3,3'-(2,4-diaminopteridine-6,7-diyl)diphenol | C18 H14 N6 O2 | 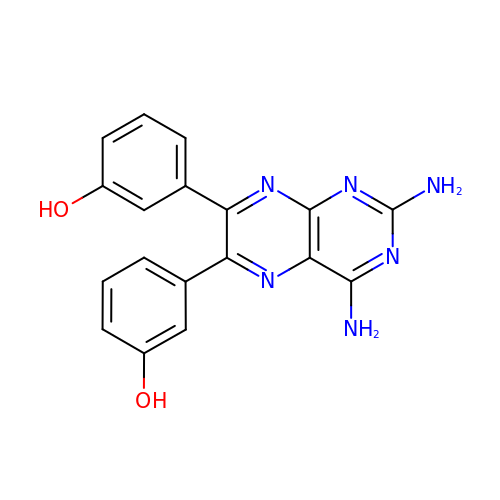UJIAQDJKSXQLIT-UHFFFAOYSA-N Cas13a are single-molecule effectors of the Class II, Type VI family of CRISPR-Cas systems that are part of the bacterial and archaeal defense systems. These RNA-guided and RNA-activated RNA endonucleases are characterized by their ability to cleave target RNAs complementary to the crRNA-spacer sequence, as well as bystander RNAs in a sequence-unspecific manner. Due to cleavage of cellular transcripts they induce dormancy in the host cell and thus protect the bacterial population by aborting the infectious cycle of RNA-phages. Here we report the structural and functional characterization of a Cas13a enzyme from the photo-auxotrophic purple bacteria Rhodobacter capsulatus.

The RcCas13a-crRNA binary complex exhibits a markedly increased stability of about 10 °C. We determined the X-ray crystal structure of the binary complex by experimental phasing, using crystals of SeMet-labeled RcCas13a protein and refined the final coordinates against data collected on native RcCas13a-crRNA complex crystals to 2.1 Å resolution (for X-ray data processing, structure solution and refinement statistics see Table 1). Protein residues as well as nucleobases of the repeat-region and the first 16nt’s of the spacer in the crRNA are well defined in the electron density. However, we did not observe electron density for the C-terminal 120 aa residues, that are unique to RcCas13a. The binary complex structure of RcCas13a shows the enzyme in a contracted, inactive conformation. Here, in the composite active site made up by the HEPN1 and HEPN2 domains, His 469 of the conserved catalytic tetrad (Arg 464 + His 469/Arg 1052 + His 1057) is shifted about 18 Å away, preventing endonuclease activity prior to target RNA binding. Thus, the stable contracted conformation of the binary complex as observed in RcCas13a, likely prevents premature activation of the RNase function. RcCas13a recognizes its ~58 nt long crRNA predominantly via shape-recognition, but makes nucleobase-specific interactions with its stem-loop and 3′ flank of the crRNA. In addition, a base-specific readout of the bulge formed by A-8 and C-7 at the 3′ base of the stem-loop occurs via bi-dental hydrogen-bonding of Arg 23 and the peptide backbone of the β-hairpin in the NTD to the Watson–Crick–Franklin face of C-7. Distinct to the crRNAs from Lba, Lbu, Lse and LshCas13a, the stem-loop in the crRNA of RcCas13a is extended by one C-G base pair and an additional 3.4 Å interaction between the twisted C-28 (3N) and G-5 (1N) at the base of the stem, next to the conserved U-A base-pair can be observed. We tested all RcCas13a mutants for their pre-crRNA cleavage activity and could identify Arg 1085, Asn 1089 and His 1113 as key residues essential for pre-crRNA processing.

>[2x]MQIGKVQGRTISEFGDPAGGLKRKISTDGKNRKELPAHLSSDPKALIGQWISGIDKIYRKPDSRKSDGKAIHSPTPSKMQFDARDDLGEAFWKLVSEAGLAQDSDYDQFKRRLHPYGDKFQPADSGAKLKFEADPPEPQAFHGRWYGAMSKRGNDAKELAAALYEHLHVDEKRIDGQPKRNPKTDKFAPGLVVARALGIESSVLPRGMARLARNWGEEEIQTYFVVDVAASVKEVAKAAVSAAQAFDPPRQVSGRSLSPKVGFALAEHLERVTGSKRCSFDPAAGPSVLALHDEVKKTYKRLCARGKNAARAFPADKTELLALMRHTHENRVRNQMVRMGRVSEYRGQQAGDLAQSHYWTSAGQTEIKESEIFVRLWVGAFALAGRSMKAWIDPMGKIVNTEKNDRDLTAAVNIRQVISNKEMVAEAMARRGIYFGETPELDRLGAEGNEGFVFALLRYLRGCRNQTFHLGARAGFLKEIRKELEKTRWGKAKEAEHVVLTDKTVAAIRAIIDNDAKALGARLLADLSGAFVAHYASKEHFSTLYSEIVKAVKDAPEVSSGLPRLKLLLKRADGVRGYVHGLRDTRKHAFATKLPPPPAPRELDDPATKARYIALLRLYDGPFRAYASGITGTALAGPAARAKEAATALAQSVNVTKAYSDVMEGRTSRLRPPNDGETLREYLSALTGETATEFRVQIGYESDSENARKQAEFIENYRRDMLAFMFEDYIRAKGFDWILKIEPGATAMTRAPVLPEPIDTRGQYEHWQAALYLVMHFVPASDVSNLLHQLRKWEALQGKYELVQDGDATDQADARREALDLVKRFRDVLVLFLKTGEARFEGRAAPFDLKPFRALFANPATFDRLFMATPTTARPAEDDPEGDGASEPELRVARTLRGLRQIARYNHMAVLSDLFAKHKVRDEEVARLAEIEDETQEKSQIVAAQELRTDLHDKVMKCHPKTISPEERQSYAAAIKTIEEHRFLVGRVYLGDHLRLHRLMMDVIGRLIDYAGAYERDTGTFLINASKQLGAGADWAVTIAGAANTDARTQTRKDLAHFNVLDRADGTPDLTALVNRAREMMAYDRKRKNAVPRSILDMLARLGLTLKWQMKDHLLQDATITQAAIKHLDKVRLTVGGPAAVTEARFSQDYLQMVAAVFNGSVQNPKPRRRDDGDAWHKPPKPATAQSQPDQKPPNKAPSAGSRLPPPQVGEVYEGVVVKVIDTGSLGFLAVEGVAGNIGLHISRLRRIREDAIIVGRRYRFRVEIYVPPKSNTSKLNAADLVRIDENLYFQKLAAALEHHHHHH> ALWQFNGMIKCKIPSSEPLLDFNNYGCYCGLGGSGTPVDDLDRCCQTQDNCYKQAKKLDSCKVLVDNPYTNNYSYSCSNNEITCSSENNACEAFICNCDRNAAICFSKVPYNKEHKNLDKKN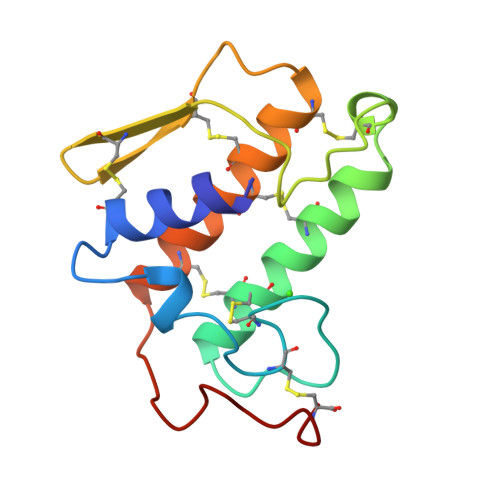C> GSTLQPLENSTRQEKLLYPKLNQLSNSINAAVAFLLEARNLEGWWQDFNFPQAASIGDEWVTAYVGTMLATLPYAHVHEALMQAWELLKIRDHRPTGEWGYNYILCGDADTTGWALQLAAAVGASDSERAQQARAALATHLQPNGGIATFAEESIRAYIKVP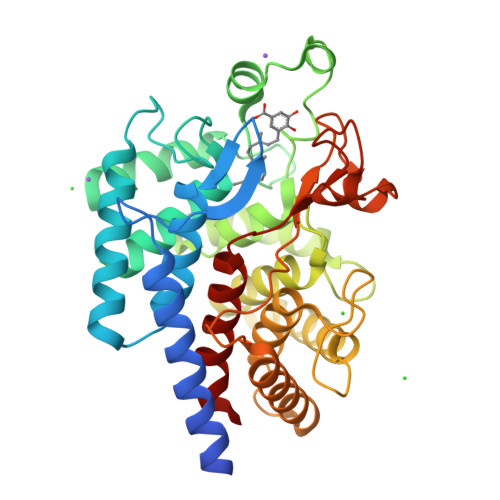DLANVSFQGWCGAHTCVSAAVAALPEFRSRLHDYLRVTQTSQGNWEGYWWSDHEYTTALTAEALAAGGQAADQPSIEQAVAWGLKRLCPQGFVATSKHPNGSTFATAWCLRLLLLNTVDAEVKAARAAAIGWLLEQQRPNGSWVSSAYLRIPYPFDRNPNQFPHWRYYDEIEGDKRFEGSIIFDHNSIFTTATVVNSLVKAAPML> MGFCLALAWTLLVGAWTPLGAQNPISWEVQRFDGWYNNLMEHRWGSKGSRLQRLVPASYADGVYQPLGEPHLPNPRDLSNTISRGPAGLASLRNRTVLGVFFGYHVLSDLVSVETPGCPAEFLNIRIPPGDPMFDPDQRGDVVLPFQRSRWDPETGRSPSNPRDPANQVTGWLDGSAIYGSSHSWSDALRSFSRGQLASGPDPAFPRDSQNPLLMWAAPDPATGQNGPRGLYAFGAERGNREPFLQALGLLWFRYHNLWAQRLARQHPDWEDEELFQHARKRVIATYQNIAVYEWLPSFLQKTLPEYTGYRPFLDPSISSEFVAASEQFLSTMVPPGVYMRNASCHFQGVINRNSSVSRALRVCNSYWSREHPSLQSAEDVDALLLGMASQIAEREDHVLVEDVRDFWPGPLKFSRTDHLASCLQRGRDLGLPSYTKARAALGLSPITRWQDINPALSRSNDTVLEATAALYNQDLSWLELLPGGLLESHRDPGPLFSTIVLEQFVRLRDGDRYWFENTRNGLFSKKEIEEIRNTTLQDVLVAVINIDPSALQPNVFVWHKGDPCPQPRQLSTEGLPACAPSVVRDYFEGSGFGFGVTIGTLCCFPLVSLLSAWIVARLRMRNFKRLQGQDRQSIVSEKLVGGMEALEWQGHKEPCRPVLVYLQPGQIRVVDGRLTVLRTIQLQPPQKVNFVLSSNRGRRTLLLKIPKEYDLVLLFNLEEERQALVENLRGALKESGLSIQEWELREQELMRAAVTREQRRHLLETFFRHLFSQVLDINQADAGTLPLDSSQKVREALTCELSRAEFAESLGLKPQDMFVESMFSLADKDGNGYLSFREFLDILVVFMKGSPEEKSRLMFRMYDFDGNGLISKDEFIRMLRSFIEISNNCLSKAQLAEVVESMFRESGFQDKEELTWED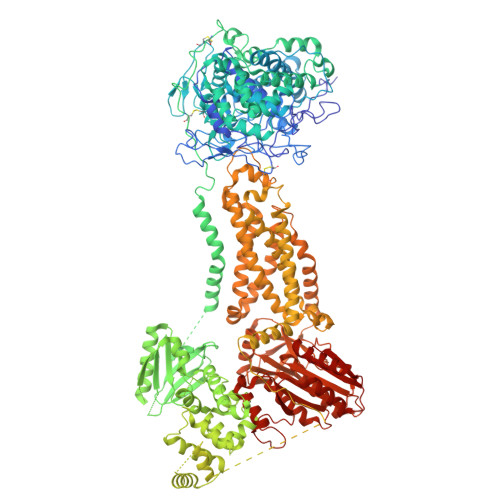FHFMLRDHNSELRFTQLCVKGVEVPEVIKDLCRRASYISQDMICPSPRVSARCSRSDIETELTPQRLQCPMDTDPPQEIRRRFGKKVTSFQPLLFTEAHREKFQRSCLHQTVQQFKRFIENYRRHIGCVAVFYAIAGGLFLERAYYYAFAAHHTGITDTTRVGIILSRGTAASISFMFSYILLTMCRNLITFLRETFLNRYVPFDAAVDFHRLIASTAIVLTVLHSVGHVVNVYLFSISPLSVLSCLFPGLFHDDGSEFPQKYYWWFFQTVPGLTGVVLLLILAIMYVFASHHFRRRSFRGFWLTHHLYILLYVLLIIHGSFALIQLPRFHIFFLVPAIIYGGDKLVSLSRKKVEISVVKAELLPSGVTHLRFQRPQGFEYKSGQWVRIACLALGTTEYHPFTLTSAPHEDTLSLHIRAAGPWTTRLREIYSAPTGDRCARYPKLYLDGPFGEGHQEWHKFEVSVLVGGGIGVTPFASILKDLVFKSSVSCQVFCKKIYFIWVTRTQRQFEWLADIIREVEENDHQDLVSVHIYITQLAEKFDLRTTMLYICERHFQKVLNRSLFTGLRSITHFGRPPFEPFFNSLQEVHPQVRKIGVFSCGPPGMTKNVEKACQLINRQDRTHFSHHYENF>[2x]AEAGITGTWYNQLGSTFIVTAGADGALTGTYESAVGNAESRYVLTGRYDSAPATDGSGT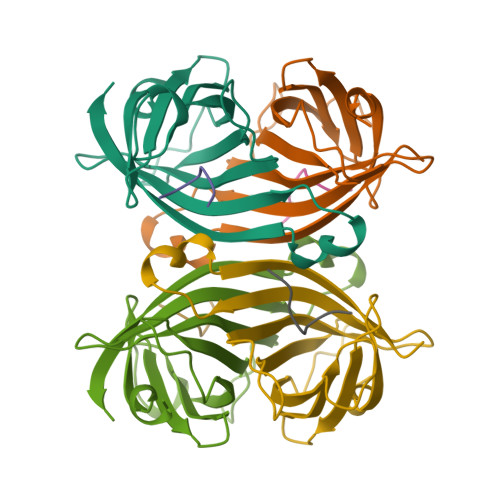ALGWTVAWKNNYRNAHSATTWSGQYVGGAEARINTQWLLTSGTTEANAWKSTLVGHDTFTKVKP;>[2x]FSHPQNT>VAQISPQYPMFTVPLPIPPVKQPRLTVTNPVNGQEIWYYEVEIKPFTHQVYPDLGSADLVGYDGMSPGPTFQVPRGVETVVRFINNAEAPNSVHLHGSFSRAAFDGW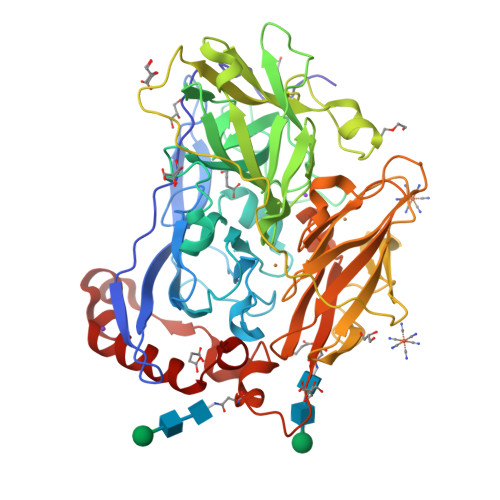AEDITEPGSFKDYYYPNRQSARTLWYHDHAMHITAENAYRGQAGLYMLTDPAEDALNLPSGYGEFDIPMILTSKQYTANGNLVTTNGELNSFWGDVIHVNGQPWPFKNVEPRKYRFRFLDAAVSRSFGLYFADTDAIDTRLPFKVIASDSGLLEHPADTSLLYISMAERYEVVFDFSDYAGKTIELRNLGGSIGGIGTDTDYDNTDKVMRFVVADDTTQPDTSVVPANLRDVPFPSPTTNTPRQFRFGRTGPTWTINGVAFADVQNRLLANVPVGTVERWELINAGNGATHPIHIHLVDFKVISRTSGNNARTVMPYESGLKDVVWLGRRETVVVEAHYAPFPGVYMFHCHNLIHEDHDMMAAFNATVLPDYGYNATVFVDPMEELWQARPYELGEFQAQSGQFSVQAVTERIQTMAEYRPYAAADE[2x]>[2x]GMIKKANKISYDEVPYPPFTFSYTYPPYLRTIGKLFGLNPPLLETAKVLDIGCGIGVNLLNFAETYPKSQSLGVDLSKTQIELGKKTISDAKINNVELKALSILDLDESYGKFDYIVCHGVYSWVSQEVQDKILEVLNKLLNPNGIAFVSYNTLPGWNMQNTIREMMMFHSESFNTSHDKLQQARLLLKFINDSLGNSTTPYANFLRDEAKLISTYDDSYVLHEYLGEINTGTYFHQFIEKAQKNHLNYLGDTSIAAMFIGNLPTKAASKLQAINDIVCTEQYMDFITNRKFRSTLLCHQNIPINRKIEFDNLKDFYTTFNIRPISPENKIDLNNEQENISFYYENLPEPFISTTSA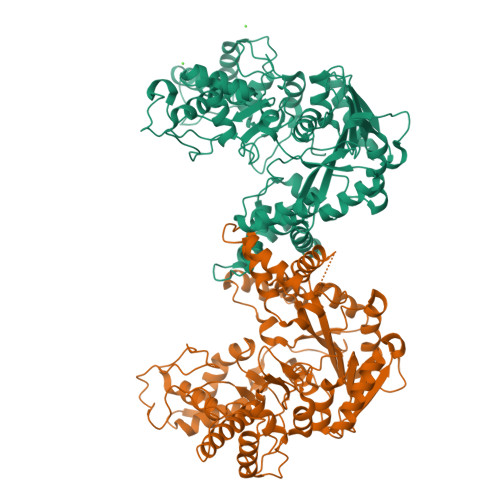IMKAILYVYAENISNPIRLEQVAKEAFKKLGKYRLQDFLATLEQHFITLIFQGYLKIFETKPHAIATITEKPKTSQFARYQAKHAHFNNVTNMFSITNRLNDMIGIPIHEKYILEMLDGTHNIDDIKKSIIEKINSKLLTACDNKGQVVTDPKLLKEFVDYVVAVSLEKFRINYLLVG>NLYFQGMIPLEQGIEFLSVNVEEDSPVVGKKLKDLPLPRDSIIAAIVRGGVLVVPRGDTEILSGDKLYVIVSAEAKETV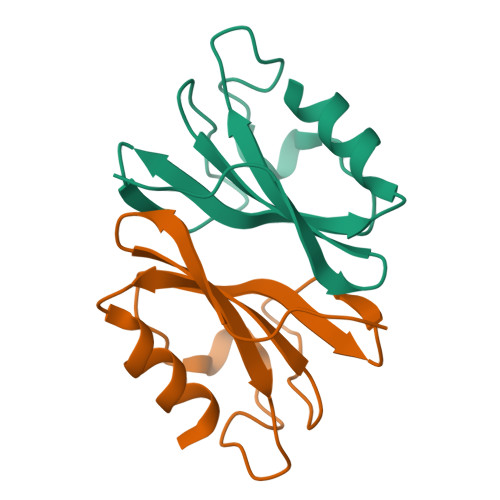EETLLGR[2x]> KDEDNLDFTKNLLTRIKNLH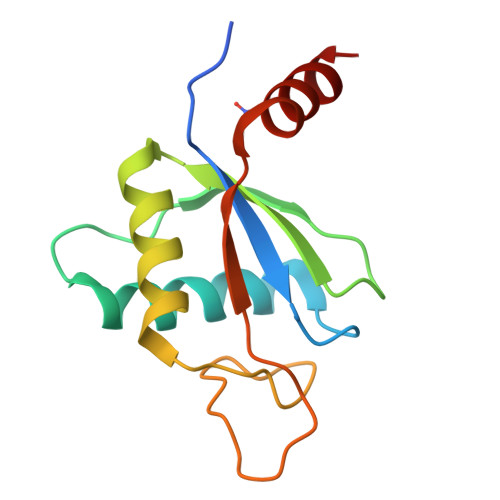PLTNKSTIHSLLSYVFSRQTQNIACEPMYIDYRKDETEAIIRWKTPLHAETCINAFRTQERKQNSHDDIRAHRKKGSSRPFLIAELITGEEEKNYWRMLKK>SSGHMRSTVFSDEEFSNILNDFPALKRNINGKRLVYLDNAASTLKCKSVIEKMTDFYLYHYSNIHRAVHTLASEATVAYEQAREKVANFLNASSEEIIFTSGTTMGINFLVNSLAKSGILKTEDTVLISQVEHHANLVPWVRLSKFYGFKVAYITADEKGVITNESILKTKESIPNPKVVSITGQSNVTGQEMPIELIRETFKNATLIVDGAQLVPHKKVDVKKLDVDFLVFSGHKILGPTGIGVLYGKKALLEQLEPFLYGGEMIDKVTFEDVTFNVLPYRFEAGTQ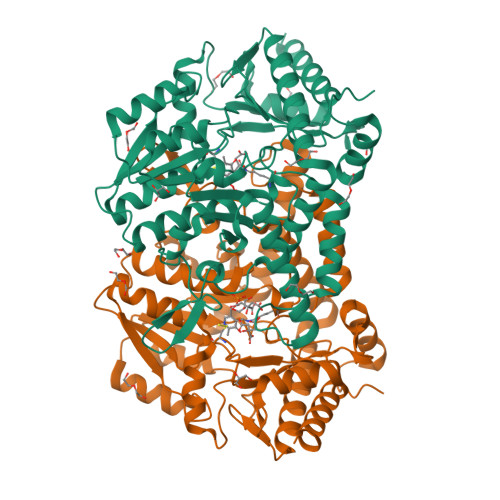HITGAVGLGYTIDYLESIGFEKVEKHVEELSNYLLEKMMELDFVEVYGPIDSSHKSLVSFNVKGVHPHDVSHILDENFGVATRSGHHCAQPLMGVLAKGSKIDFPNSTVRASVYLYNTKEDIDVLIEGLKYIRRWFE[4x]The pilin subunits of GBS are assembled into high molecular weight polymers via a transpeptidation reaction catalyzed by specific pilin-associated class C sortases, through a common mechanism involving specific motifs present in the pilin proteins. The pilin-related sortases, which are integral membrane cysteine transpeptidases, cleave the LPXTG-like motif of the pilin proteins and, via the Thr residue, covalently join the C-terminus of one pilin subunit to a Lys side chain (ε amino group) on the next subunit. In this work, we present the high-resolution crystal structures of SrtC2 and SrtC1 from GBS PI-1.

The overall fold of GBS PI-1 SrtC2 is similar to SrtC1, with a root-mean-square deviation (rmsd) of 0.94 Å for 169 aligned Cα atoms. Like SrtC1, SrtC2 is predicted to form two N-terminal α-helices; absence of electron density for the first α-helix of SrtC2 is likely an artifact of crystallization that may be due constraints imposed by crystal packing or simply to local disorder in this N-terminal region of the structure, as commonly observed in crystal structures. The His156, Cys218, Arg227 catalytic triad in SrtC2 is conserved in spatially equivalent positions in all sortase enzymes. In GBS SrtC2 and SrtC1, the conserved catalytic His in the β4-α4 loop interacts indirectly with the catalytic Cys through the formation of a water-mediated hydrogen bond. The side-chain carboxylate group of Asp84 in the lid of SrtC2 makes a salt bridge with the side chain of the conserved catalytic Arg227, and the ring of Phe86 interacts with Thr154 in a hydrophobic pocket made of conserved residues. The pyrollidine ring of the conserved Pro85 in the lid also interacts with this hydrophobic pocket. The aromatic ring of Phe86 in SrtC2 forms an aromatic-sulfur interaction with the catalytic Cys that has been previously observed in other pilus-related sortases. Surprisingly, the ligand-free SrtC structures matched the active, peptide-bound, conformation of S. aureus SrtA better than that of apo-SrtA. In both enzymes, the catalytic residues are not accessible to pilin substrates, suggesting that the enzymes cannot bind substrates in this conformation.

> ASHQNINQFKREVAKIDTNTVERRIALANAYNETLSRNPLLIDPFTSKQKEGLREYARMLEVHEQIGHVAIPSIGVDIPIYAGTSETVLQKGSGHLEGTSLPVGGLSTHSVLTAHRGLPTARLFTDLNKVKKGQIFYVTNIKETLAYKVVSIKVVDPTALSEVKIVNGKDYITLLTCTPYMINSHRLLVKGERIPYDSTEAEKHKEQTVQDYRLS>[2x]MKKWIRNGTVVTASDTYQADVLIDGEKVVAIGSDL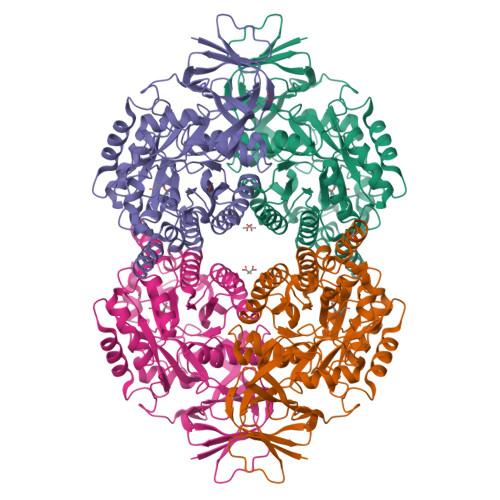QATDAEVIDATGYYLLPGGIDPHTHLDMPFGGTVTSDNFFTGTKAAAFGGTTSIVDFCLTSKGESLHSAIATWHEKARGKAVIDYGFHLMVSDANDHVLEELESVVNNEGITSLKVFMAYKNVLMADDETLFKTLIRAKELGALVQVHAENGDVLDYLTKQALAEGNTDPIYHAYTRPPEAEGEATGRAIALTALADAQLYVVHVSCADAVRRIAEAREKGWNVYGETCPQYLVLDITALEKPDFEGAKYVWSPPLREKWNQDVLWSALKNGILQTVGSDHCPFNFSGQKELGRRDFTKIPNGGPIIEDRMTILFSEGVRKGKISLNQFVDITSTKVAKLFGMFPQKGTIAVGSDADIVLFDPTVQRTISVETHHMNVDYNPFEGMQVHGDVISVLSRGAFVVRNKQFVGHAGAGRYVKRSTFARP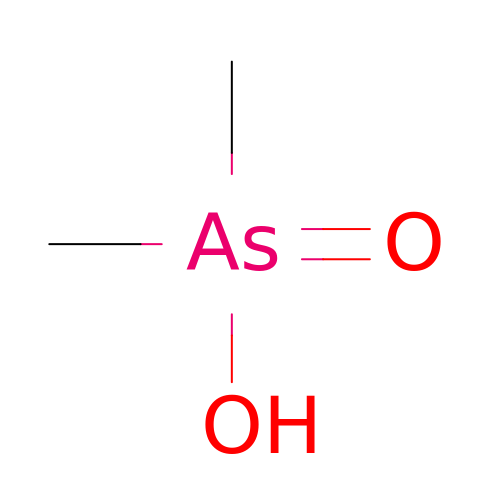CACODYLIC ACID | C2 H7 As O2 | OGGXGZAMXPVRFZ-UHFFFAOYSA-N4-[[[6-[(4,4-dimethylpiperidin-1-yl)methyl]pyridin-3-yl]amino]methyl]-1-[6-[(phenylmethyl)amino]pyrimidin-4-yl]piperidin-4-ol | C30 H41 N7 O | 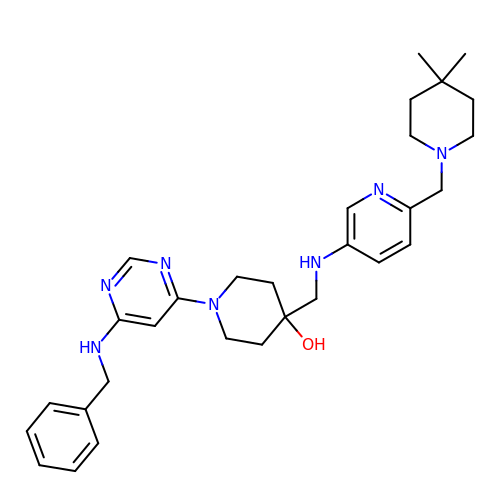GTLDMCHZRAFXCB-UHFFFAOYSA-N>MKITAARVIITCPGRNFVTLKIETDQGVYGIGDATLNGRELSVVAYLQEHVAPCLIGMDPRRIEDIWQYVYRGAYWRRGPVTMRAIAAVDMALWDIKAKMAGMPLYQLLGGRSRDGIMVYGHANGSDIAETVEAVGHYIDMGYKAIRAQTGVPGIKDAYGVGRGKLYYEPADASLPSVTGWDTRKALNYVPKLFEELRKTYGFDHHLLHDGHHRYTPQEAANLGKMLEPYQLFWLEDCTPAENQEAFRLVRQHTVTPLAVGEIFNTIWDAKDLIQNQLIDYIRATVVGAGGLTHLRRIADLASLYQVRTGCHGATDLSPVTMGCALHFDTWVPNFGIQEYMRHTEETDAVFPHDYWFEKGELFVGETPGHGVDID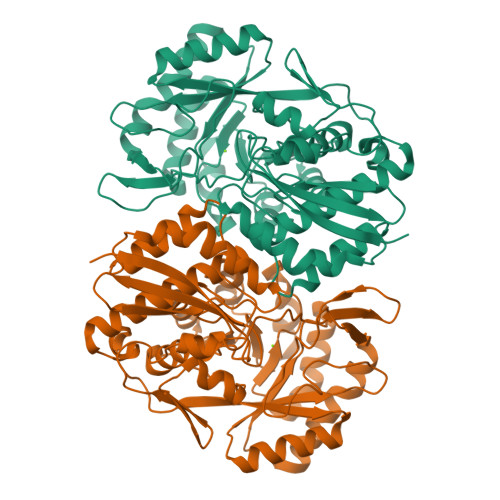EELAAKYPYKPAYLPVARLEDGTMWNW[4x]>[3x]ATPHNSAQVGDFAETVLMCGDPLRAKLIAETYLENPKLVNNVRGIQGYTGTYKGKPISVMGHGMGLPSICIYAEELYSTYKVKTIIRVGTCGAIDMDIHTR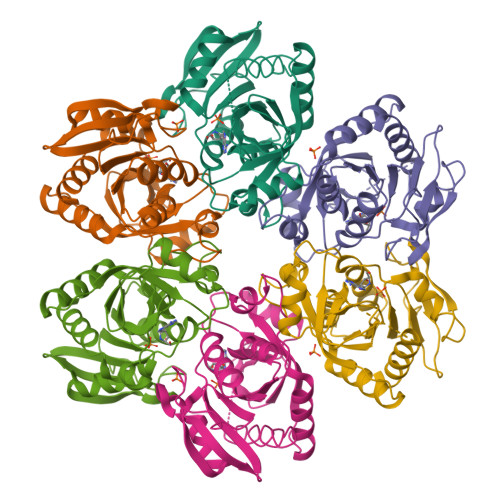DIVIFTSAGTNSKINRIRFMDHDYPATASFDVVCALVDAAKELNIPAKVGKGFSTDLFYNPQTELAQLMNKFHFLAVEMESAGLFPIADLYGARAGCICTVSDHILHHEETTAEERQNSFQNMMKIALEAAIKLH alpha-(4-pyridyl-1-oxide)-N-tert-butylnitrone 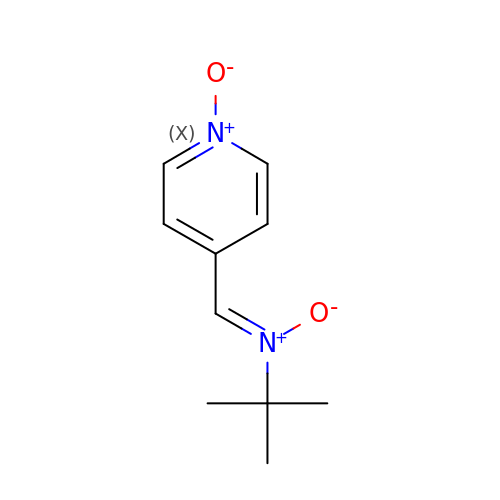| C10 H14 N2 O2 | RNRMWTCECDHNQU-WQLSENKSSA-N> MTNAMKVEGYPSMEWPTSLDIPLKASEELVGIDLETDLPDDPTDLKTLLVEENSEKEHWLTIALAYCNHGKTNEGIKLIEMALDVFQNSERASLHTFLTWAHLNLAKGQSLSVETKEHELTQAELNLKDAIGFDPTWIGNMLATVELYYQRGHYDKALETSDLFVKSIHAEDHRSGRQSKPNCLFLLLRAKLLYQKKNYMASLKIFQELLVINPVLQPDPRIGIGLCFWQLKDSKMAIKSWQRALQLNPKNTSASILVLLGEFRESFTNSTNDKTFKEAFTKALSDLNNIFSENQHNPVLLTL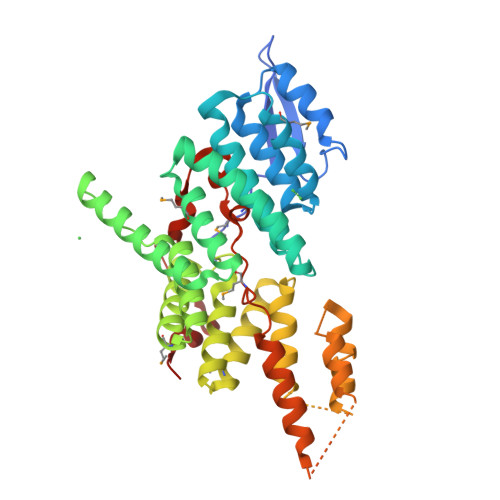LQTYYYFKGDENLYFQSETNADSSQLINSLYIKTNVTNLIQQDEDLGMPVDLMKFPGLLNKLDSKLLYGFDNVKLDKDDRILLRDPR> MAIIYNPNKKIFTLHTAHTTYQMQVDPLGYLLHLYYGEKTNSSMDYVL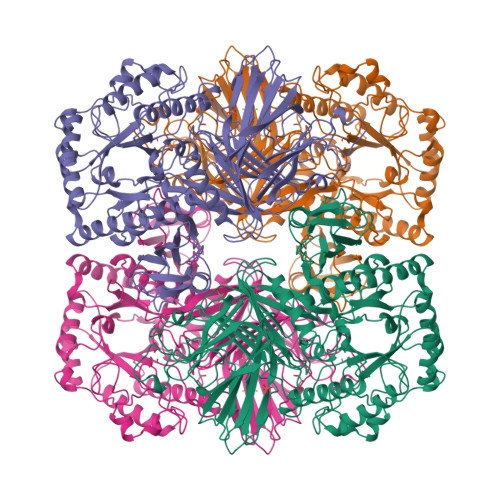TYADRGFSGNPYAAGMDRTYSLDALPQEYPSLGTGDYRNIALNIKNEKGVESADLLFKSYEIRNGKYRLQGLPAVWADEKEAQTLEIVLADENAQVEVHLLYGVLEENDVITRSVRIKNTGTGQITIEKAAAACLDFVQGEFDVLRFYGKHAMERNLERTPLGHGTIAFGSRRGTSSHQYNPAVILAEKGTTETAGSCYGMLFVYSGNFSCEAEKDQFNQTRLLLGLNEELFSYPLASGETFTVPEVILSYSAEGLSALSQQYHNCIRNHVCRSKYVHMQRPVLINSWEAAYFDFTGDTIVDLAKEAASLGIDMVVMDDGWFGKRNDDNSSLGDWQVNETKLGGSLAELITRVHEQGMKFGIWIEPEMINEDSDLYRAHPDWAIRIQGKKPVRSRNQLLLDFSRKEVRDCVFDQICVVLDQGKIDYVKWDMNRSMADVYAGNLSYDYVLGVYDFMERLCSRYPDLLLEGCSGGGGRFDAGMLYYSPQIWCSDNTDAINRTRIQYGTSFFYPVSAMGAHVSAVPNHQTGRVTSFHTRGVTAMAGTFGYELNPALLSDEEKQQIREQIKTYKKYETLINEGTYWRLSDPFTDEIAAWMSVSEEQDHALVSVVRLMAEANQATVYVRLRGLKPDAVYLEEQSGRQYSGAALMHAGIPLPPFTEEYEAYQFAFTEL>[2x]GTDDATADSRKTYTLTDYLKNTYRLKLYSLRWISDHEYLYKQENNILVFNAEYGNSSVFLENSTFDEFGHSINDYSISPDGQFILLEYNYVKQWRHSYTASYDIYDLNKRQLITEERIPNNTQWVTWSPVGHKLAYVWNNDIYVKIEPNLPSYRITWTGKEDIIYNGITDWVYEEEVFSA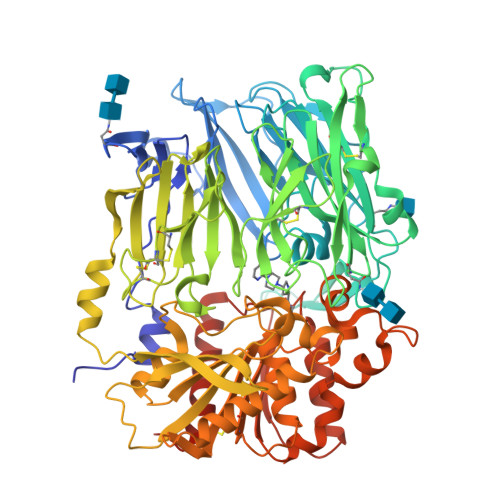YSALWWSPNGTFLAYAQFNDTEVPLIEYSFYSDESLQYPKTVRVPYPKAGAVNPTVKFFVVNTDSLSSVTNATSIQITAPASMLIGDHYLCDVTWATQERISLQWLRRIQNYSVMDICDYDESSGRWNCLVARQHIEMSTTGWVGRFRPSEPHFTLDGNSFYKIISNEEGYRHICYFQIDKKDCTFITKGTWEVIGIEALTSDYLYYISNEYKGMPGGRNLYKIQLSDYTKVTCLSCELNPERCQYYSVSFSKEAKYYQLRCSGPGLPLYTLHSSVNDKGLRVLEDNSALDKMLQNVQMPSKKLDFIILNETKFWYQMILPPHFDKSKKYPLLLDVYAGPCSQKADTVFRLNWATYLASTENIIVASFDGRGSGYQGDKIMHAINRRLGTFEVEDQIEAARQFSKMGFVDNKRIAIWGWSYGGYVTSMVLGSGSGVFKCGIAVAPVSRWEYYDSVYTERYMGLPTPEDNLDHYRNSTVMSRAENFKQVEYLLIHGTADDNVHFQQSAQISKALVDVGVDFQAMWYTDEDHGIASSTAHQHIYTHMSHFIKQCFSLPLVPRGSHHHHHH> MTTLLNPYFGEFGGMYVPQILMPALNQLEEAFVSAQKDPEFQAQFADLLKNYAGRPTALTKCQNITAGTRTTLYLKREDLLHGGAHKTNQVLGQALLAKRMGKSEIIAETGAGQHGVASALASALLGLKCRIYMGAKDVERQSPNVFRMRLMGAEVIPVHSGSATLKDACNEALRDWSGSYETAHYMLGTAAGPHPYPTIVREFQRMIGEETKAQILDKEGRLPDAVIACVGGGSNAIGMFADFINDTSVGLIGVEPGGHGIETGEHGAPLKHGRVGIYFGMKAPMMQTADGQIEESYSISAGLDFPSVGPQHAY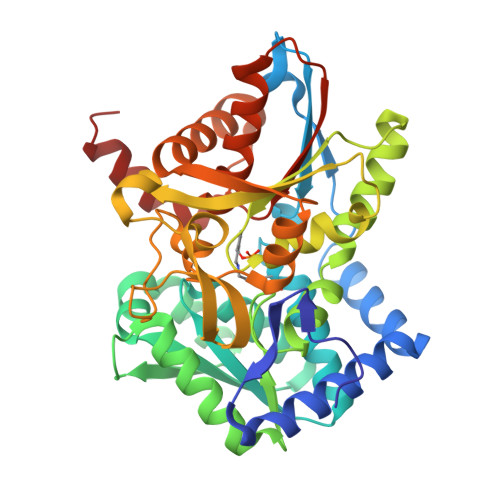LNSIGRADYVSITDDEALEAFKTLCRHEGIIPALESSHALAHALKMMREQPEKEQLLVVNLSGRGDKDIFTVHDILKARGEI> HHHHHHSSGLVPRGSHMQTTTVYSLEDLLPYLKQDNVDVKLAPGTYNVNGFDVGEDRLFSTTPLFLFEGSNSTYDFTDVKLNINTVVLTKFGNNEVNEIQILGNNNVLKNLKLEDIGTTAPSNRAQSIVIDGRDNRIEGFHLTIRGSYPYGYGDAFGAGGGSVINHRKHSGVLIRGLRNHLKDCTIISRSYGHIVFMQAASY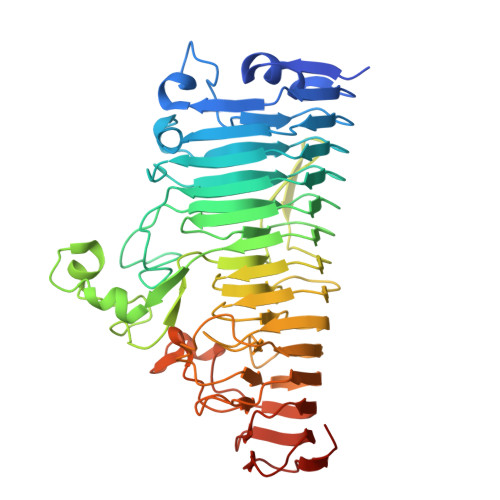PTVEGCYIEGEMRSTDDMLAEEGTGSPADKVDFMTVWGYKLPAGYMMSLQEGGIRAYNAGTTYIDGVEIQRATDNPTVLNCTIKNARTGVTLAHANGTKYVEGCTVLGCENGYSIGSGTVVNCGADAIYGPVFKNTYGSDKGYNADITILPPSDAYYNGHDAVAYIGGSNHNLTFRSEITEIPSNLKIMVSGDLQGLRVLHGSNPSQNNFAGTNIVLRNLTNFPVDLHSDSSNITVTSCDTDNITDNGTNNSIEAIDCDSD> GNFRIKPPGARHAFPKLGTHRMVMFRRMNLLNWPPEDASPLHPIEPWGRQFFVFNAFATIDPADWCGPRGPFPRLPPLAKPAPDAATL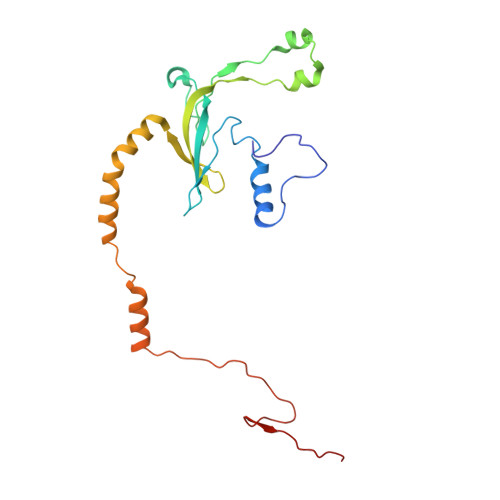AASPSSLLSALRETEERSATRTVMCVTDFAQRPLMFLGKDDFRALRENLPRIKEELKAFKERIQPNPVHAQYDLRRKLLVYPRQAMQRLKTGEHGGYGTRRGTIRERKT> HPICEVSKVASHLEVNCDKRDLTALPPDLPKDTTILHLSENLLYTFSLATLMPYTRLTQLNLDRCELTKLQVDGTLPVLGTLDLSHNQLQSLPLLGQTLPALTVLDVSFNRLTSLPLGALRGLGELQELYLKGNELKTLPPGLLTPTPKLEKLSLANNDLTELPAGLLNGLENLDTLLLQENSLYTIPKGFFGSHLLPFAFLHGNPWLCNCEILYFRRWLQ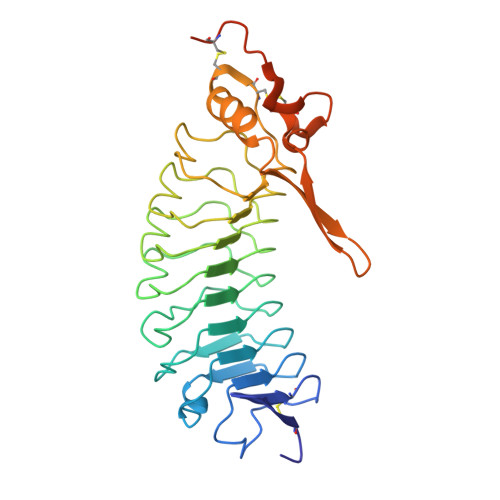DNAENVYVWKQGVDVKAMTSNVASVQCDNSDKFPVYKYPGKGCPTLGDEGDTDLYDYYPEEDTEGDK> SNAPRRSIHLSNIVEQRVFEDDEIISTPKRGRSKKTVQDNDEDYSPKKSVQKTPTRTRRSSTTTKTATTPSKGITTATATPMTPSQKMKKIRAGELSPSMQQRTDLPAKDSSKSELQLAREQLHVSVVPKSLPCREREFENIYAFLEGKIQDQCGGCMYVSGVPGTGKTATVTGVIRTLQRMAKQNELPAFEYLEINGMRLTEPRQAYVQIYKQLTGKTVSWEQAHALLEKRFTTPAPRRVTTVLLVDELDILCNRRQDVVYNLLDWPTKSAAKLVVVTIANTMDLPERLLMGKVTSRLGLTRLTFQPYSHKQLQEIVTARLGGSETFKGEAVQLVARKVAAVSGDARRALDICRRATEIADTAAVKCVTM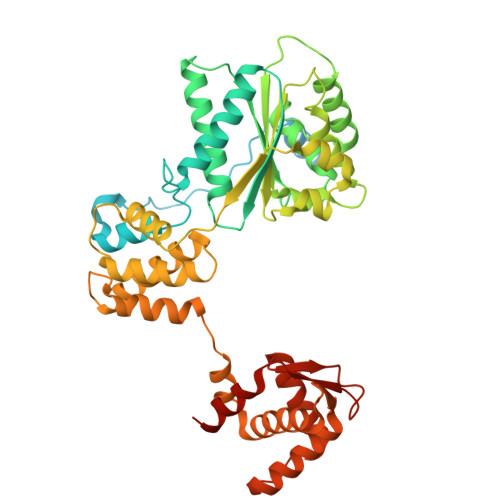LHVQQALAEMIASAKVQAIRNCSRMEQIFLQAIAAEVTRTGVEETTFMGVYQQVETIAAFMGVTFPPPGRALRLCSKLGAERLIISEHSRNDLFQKILLNVSADDIHYALRVEEMVN>SNPRLTKVLDEMSKKPCVNINEIRKMIRNFQPQFIQPRNGNRPNAQPRTVDSFEWVVRIQSTVETQLLGATNTVPQQTLNLDISFTDDSTTITPASIPGSISMLDNSRHIPAIQSMIQNFKARYLGSLQDTAQLQSPQYPQLLAYLFGQLIAIKDRLDLFRPSNPLSLADALFGFTLAQNARPRYDDHRHAKACQGPLVIPAATNSDCGPCGFVQINANQGLTLPLGACLFVNPETVNDQSFQDFLWLIFATHHRMPNQMQNNWPFSLNIVSTCAAPGRQAPHAGELTDERVRLALDTGHRILLSMFNDDEETLRYYQRKGIETMFRPCCFYTEGGLLRKATRYVSMVPLNGLYYYNGATSYVVSPIHTDAHPGITAAIESFVDIMVLQAVFSFSGPKVVAAKVNASQIDAAMVFGPAVAEGDGFVYDPLRPAPPLSAFYTEFIHRPAEQRIFQMAMSQIYGSHAPLIIANVINSIHNCKTKIVNNKLRATFVRRPPGAPHLKADTAIINRFHDPELAYALGILADGIAPLDGSHEYNVLDELDYLFNGGDIRNCFGLNALNTRGLGQIVHIRPKREPGKRPRRGFYTTLDGQVHPVTQDAPLDEIYHWRDHGNLTRPYSCHILDSQGLEFADVSNGRSRGKILVVVNSPLKTCAAYQGPSFAPK[2x]

Clinical Tv isolates are frequently found infected with one or more strain of the double-stranded RNA (dsRNA) Trichomonas vaginalis viruses (TVVs), belonging to the Trichomonasvirus genus within totiviruses. Here, we have determined the structure of TVV2 by cryo-electron microscopy (cryoEM) at 3.6 Å resolution and derived an atomic model of its capsid. TVV2 has an icosahedral, T = 2*, capsid comprised of 60 copies of the icosahedral asymmetric unit (a dimer of the two capsid shell protein [CSP] conformers, CSP-A and CSP-B), typical of icosahedral dsRNA virus capsids. Among totiviruses, the single capsid layer is responsible for protecting and sequestering the viral genome while facilitating RdRp activity and the egression of viral mRNA into the cytosol.

From 2,034 micrographs, 2,493 particles were boxed and used for icosahedral reconstruction of the viral capsid to 4 Å, based on the 0.143 “gold-standard” Fourier shell correlation coefficient (FSC). Like other totiviruses, the TVV2 viral capsid exhibits a T = 2* icosahedral capsid shell and measures ∼430 Å across at its widest near the I5 vertices, down to ∼350 Å at its narrowest between the icosahedral 2-fold (I2) symmetry axes. The TVV2 capsid is composed of 60 IAUs, organized into 12 decameric units centered about the I5 vertices, enclosing the viral genome. Within these decamers, five CSP-As are seated nearest the I5 vertex, crowding out five CSP-Bs which sit partially intercalated between the flanking CSP-As while extending between 5-fold axes to contact CSP-Bs from two other decamers forming the icosahedral 3-fold (I3) symmetry axes. The CSP-pair, A1B1, represents a reasonable initial species formed within the cytosol, as it buries the greatest surface area between subunits (∼1,540 Å2). Additionally, the interface between the possible tetrameric intermediate, A1B1-A3B3 (∼2,525 Å2), is ∼56% larger than the alternative A1B1-A2B2 tetramer (1,619 Å2) and ∼80% larger than the A1B2-A4B3 tetramer (∼1,405 Å2), suggesting that the first may be more stable and therefore more abundant in the cytosol. The protruding loop from the floor of the dimerization domain (residues 610 to 620) appears rich in positively charged residues (R612, R617, K616, R619, and R620) and inserts into a negatively charged pocket between the carapace and dimerization domains of tetramer subunits. This insertion may act as an anchor to stabilize the association of the capsid decamers through electrostatic interactions, protecting the viral genome in place of more robust interlocking strategies. The interior capsid surface appears predominantly electronegative (red) with discrete electropositive regions (blue) including the protruding loop of the dimerization domain and residues along α1 nearer the I5 vertices. The TVV2 capsid displays similar T = 2* symmetry but does not exhibit comparable subunit interactions and instead seems to rely on the abutting interface between the CSP conformers.>[4x]SGLVPRGSHMNMQDAYFGSAAELDAVNEMLAAIGESPVTTLDEDGSADVANARRILNRINRQIQSKGWAFNINESATLTPDVSTGLIPFRPAYLSILGGQYVNRGGWVYDKSTGTDTFSGPI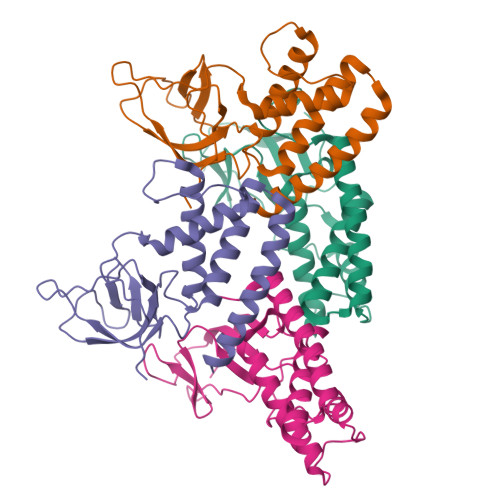TVTLITLQDYDEMPECFRQWIVTKASRQFNSRFFGAEDVENSLAQEEMEARMACNEYEMDFGQYNMLDGDAYVQGLIGR> MHHHHHHAAACERALQYKLGDKIHGFTVNQVTSVPELFLTAVKLTHDDTGARYLHLAREDTNNLFSVQFRTTPMDSTGVPHILEHTVLCGSQKYPCRDPFFKMLNRSLSTFMNAFTASDYTLYPFSTQNPKDFQNLLSVYLDATFFPCLRELDFWQEGWRLEHENPSDPQTPLVFKGVVFNEMKGAFTDNERIFSQHLQNRLLPDHTYSVVSGGDPLCIPELTWEQLKQFHATHYHPSNARFFTYGNFPLEQHLKQIHEEALSKFQKIEPSTVVPAQTPWDKPREFQITCGPDSFATDPSKQTTVSVSFLLPDITDTFE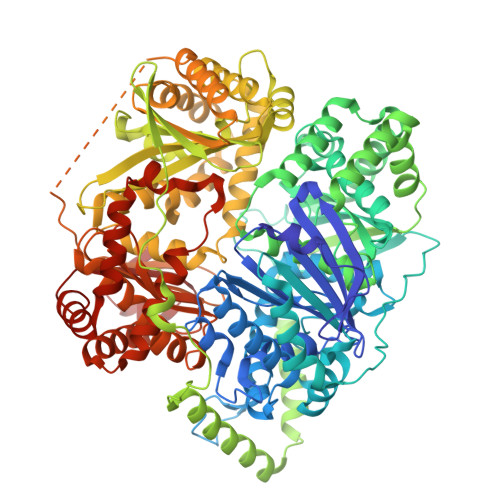AFTLSLLSSLLTSGPNSPFYKALIESGLGTDFSPDVGYNGYTREAYFSVGLQGIVEKDIETVRSLIDRTIDEVVEKGFEDDRIEALLHKIEIQMKHQSTSFGLMLTSYIASCWNHDGDPVELLKLGNQLAKFRQCLQENPKFLQEKVKQYFKNNQHKLTLSMRPDDKYHEKQAQVEATKLKQKVEALSPGDRQQIYEKGLELRSQQSKPQDASCLPALKVSDIEPTIPVTELDVVLTAGDIPVQYCAQPTNGMVYFRAFSSLNTLPEELRPYVPLFCSVLTKLGCGLLDYREQAQQIELKTGGMSASPHVLPDDSHMDTYEQGVLFSSLCLDRNLPDMMQLWSEIFNNPCFEEEEHFKVLVKMTAQELANGIPDSGHLYASIRAGRTLTPAGDLQETFSGMDQVRLMKRIAEMTDIKPILRKLPRIKKHLLNGDNMRCSVNATPQQMPQTEKAVEDFLRSIGRSKKERRPVRPHTVEKPVPSSSGGDAHVPHGSQVIRKLVMEPTFKPWQMKTHFLMPFPVNYVGECIRTVPYTDPDHASLKILARLMTAKFLHTEIREKGGAYGGGAKLSHNGIFTLYSYRDPNTIETLQSFGKAVDWAKSGKFTQQDIDEAKLSVFSTVDAPVAPSDKGMDHFLYGLSDEMKQAHREQLFAVSHDKLLAVSDRYLGTGKSTHGLAILGPENPKIAKDPSWIIR>[2x]MELRVGNRYRLGNKIGSGSFGDIYLGTDIAAGEEVAIKLECVKTKHPQLHIESKIYKMMQGGVGIPTIRWCGAEGDYNVMVMELLGPSLEDLFNFCSRKFSLKTVLLLADQMISRIEYIHSKNFIHRDVKPDNFLMGLGKKGNLVYIIDFGLAKKYRDARTHQHIPYRENKNLTGTARYASINTHLGIEQSRRDDLESLGYVLMYFNLGSLPWQGLKAATKRQKYERISEKKMSTPIEVLCKGYPSEFATYLNFCRSLRFDDKPDYSYLRQLFRNLFHRQGFSYDYVFDWNMLKF

Recently, interest in specifically targeting members of the casein kinase 1 (CK1) family, a highly conserved ubiquitously expressed serine/threonine protein kinase family, has increased enormously. The seven mammalian isoforms CK1α, β, γ1, γ2, γ3, δ and ε and their various splice variants are all highly conserved within their kinase domains (~290 residues), but differ significantly within their regulatory N-terminal and C-terminal domains. CK1 isoforms phosphorylate many different substrates bearing either a canonical or a non-canonical consensus sequence. They are involved in the regulation of many different cellular processes such as canonical Wnt signaling, DNA damage response, cell cycle progression, apoptosis and chromosome segregation (Cheong and Virshup 2010; Price 2006; Knippschild et al. 2005a, b).

In this study we identified two heterocyclic compounds (5 and 6) as potent and specific inhibitors of CK1δ (IC50 = 0.040 and 0.042 μM, respectively). Selected compound 5 was screened over 442 kinases identifying 5 as a highly potent and selective inhibitor of CK1δ. The sidechain conformation of gatekeeper methionine 82 is more compact to accommodate the trifluoromethyl-group but no deeper/selectivity pocket is opened. Hinge residues leucine 84 and leucine 85 are hydrogen bonded via the backbone carbonyl to NH and the backbone nitrogen to the imidazole nitrogen of compound 5, respectively. CH/π-bonds are formed for all three aromatic regions of compound 5. Hydrophobic interactions exist between the trifluoromethoxy-group and the sidechains of proline 87, leucine 92, phenylalanine 95, leucine 293 and phenylalanine 295. Furthermore, three crystal water molecules are found near compound 5 saturating hydrogen bond functions of the ligand and the protein surface. These water molecules are all solvent exposed and should therefore have no influence on the binding mode. According to our predictions and X-ray models, the tested compounds are not occupying the selectivity pocket.> MGRLATSPLKFPGKLAIDTLNNRLFISDSNHNRIIVTDLEGNFIVQIGSSGEEGFQDGSFEDAAFNRPQGLAYNAKKNLLYVADTENHALREIDFVNERVQTLAGNGTKGSDYQGGRKGTKQLLNSPWDVCFEPVNEKVYIAMAGQHQIWEYSVLDGITRVFSGNGYERNLNGSTPQTTSFAQPSGISLGPDLKEAYIADSESSSIRALDLQTGGSRLLAGGDPYFSENLFKFGDNDGVGAEVLLQHPLGVLCANDGQIYLTDSYNHKIKKLDPVTKRVVTLAGTGKAGFKDGKVKGAQLSEPAGLAITENGRLFVADTNNSLIRYIDLNKGEDSEILTLELKGVQPPTPKAKSLKRLRKRASADTKIVKVDSVTSREGDLNLKISLPDGYHFSKEARSKF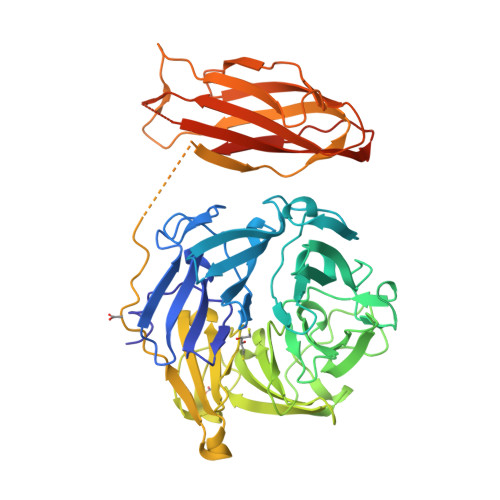VVDVEPENAVAIDPTEGTLSPEGSTMLHFIQSSTSASVGKISCKVYYCKEDEVCLYQSVQFEVPFKVESELSASPTITFTVTPRAPDAGGLQLQGTR>SNAAEPDSNRLAGEPSAYLRQHANNPVHWQPWGRKALDAAKELDRPILLSIGYAACHWCHVMAHESFEDDDVAAVMNAFFINVKVDREERPDIDQIYMAALGAMGQQGGWPLTMFLRPDGKPFWGGTYIPRHARHNMPGFVDILHAVNNLWHRDKDKINHNAEAVFDHLEGRLAAQSQPLQNEISRFDDLANRIGSLIDPQRGGIEGVPKFPNAPFMDTLWLSWLYRHNETHRDNFLLSLKTMLQGGIYDHLGGGLCRYSTDAEWLVPHFEKMLYDNAQFIRHANYAFAETGDDLFRIRIEETVDWLIREMQLPDGCFASSLDADSEGEEGKFYVWTEDEIDAVLGTDAEVFKTFYAVTPGGNWEGKNILNRLHAAAETPTPPPLVEAARRKLLAHRETRIRPGRDDKALTDWNGLAIRALAEAGRSFARTDWLEHAVQAYQSIGSSFQDGRIAHCRMEGAFLYPALATDYAAMINAALALYEATGEFAYIDDARKFKRALDGSHRDSAGNYRLSALGADDVILHAYGDYDEAIPSATSQIIEALTRLFLATGDSALYEENEKLIEQALGRALAQQYGQIGILNACRFAGEPLSLL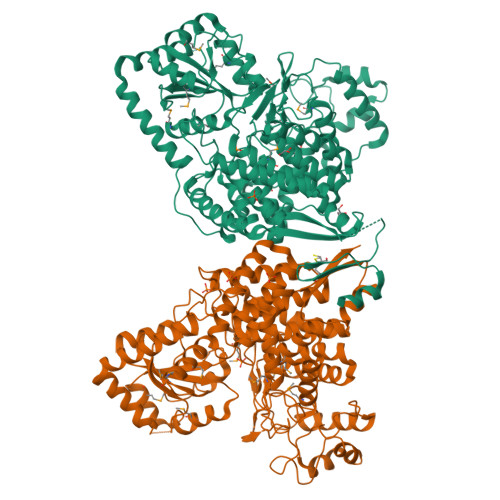IAATDRTDELVSIANRTPDPRRLDKFVLVERGKTMSLPTGGTIEPEHPAAWFCKGHVCLPPVDTGEALRSLL[2x]> MTTPVSPSPSGIIPAQLGFLAIYNPALGTTDETLEDQIVYYATASTLSQARRRHRRPRRRDRQRAQSVVKDSRPNAAGATGDSEAVAEDKDPVSKEERHERLRQIGLAQGMVEFAKSFSDGEPVDTIDTEKARVILVEVEEGWWILASIDLTRLPLPQIKTPTSSSAPPPAPNLNPLPPEPAYEYSSREVKPPSLLRADLLRAYDLFLLHHGSSLSSLLASQGRAQLVASLTRFWDHFLATWNVLLHGNPACDVFGGIKLAASGELGIGVGEEERGSGEREVLEGLVERVEGLVDVVVGRYGGPPSEKGPEEEQWLGLGGEVGEEDGAVFLGVGALDRKSLRGVVQWMEEVYVWGENAFGKPRRDLSTGHFLLGLSECSEEELTSSQANPKAIFVELKPSYQHPSRKIPPEDPQPLGKVGPELPRDHTARLRPVIYVSQPFIYILLFSEI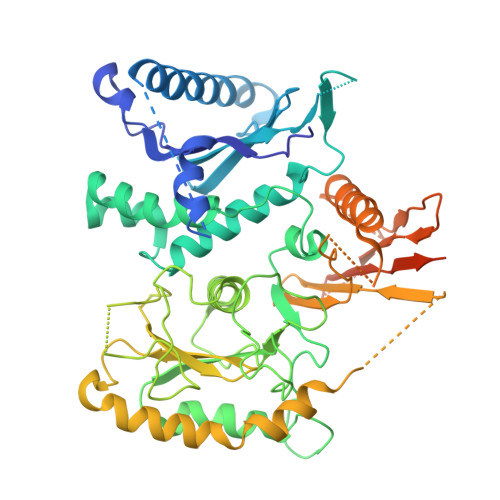TPSPSTWPTLAESLHAQLSPLQKPLLHSTSYRPERPVVETTSSSGTTTQHQIFDLVYDTETLTLQSTIPNIPDPFPYSATTPTGHSTGQQHHQQSIWTRVEALQTHAQILAILSSGRAIPTDPSSFTHLPWEEGERTCKTARGWWIVWTRVVEHSPPDAVSLHHARDDDDNDDDASCSVLGHLRSVSSSHAAGSTSSSSGSGFGLGAIPGLGGLGGWAADGATRLAQGIGIDTRRYVEGLLTSLGR> GG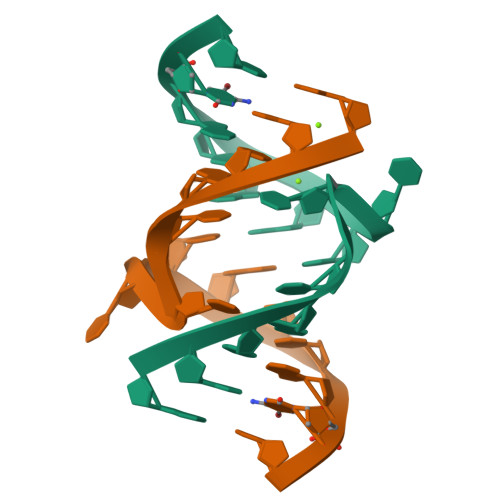UAUUUCGGUACC;> GGUAUUUUGGUACC> GLGQMLESMIDNTVRETVGAAT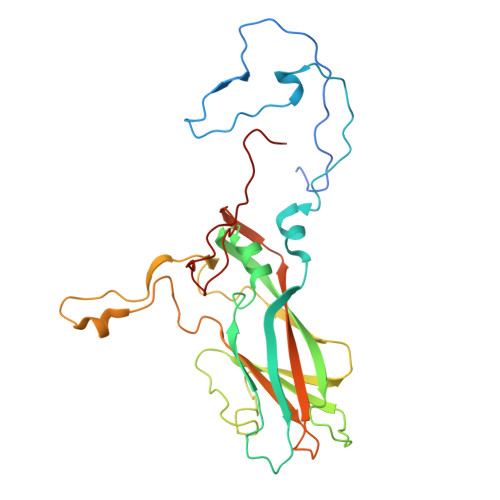SRDALPNTEASGPTHSKEIPALTAVETGATNPLVPSDTVQTRHVVQHRSRSESSIESFFARGACVTIMTVDNPASTTNKDKLFAVWKITYKDTVQLRRKLEFFTYSRFDMELTFVVTANFTETNNGHALNQVYQIMYIPPGAPVPEKWDDYTWQTSSNPSIFYTYGTAPARISVPYVGISNAYSHFYDGFSKVPLKDQSAALGDSLYGAASLNDFGILAVRVVNDHNPTKVTSKIRVYLKPKHIRVWCPRPPRAVAYYGPGVDYKDGTLTPLSTKDLTTY>MPTFLLVNDDGYFSPGINALREALKSLGRVVVVAPDRNLSGVGHSLTFTEPLKMRKIDTDFYTVIDGTPADCVHLGYRVILEEKKPDLVLSGINEGPNLGEDITYSGTVSGAMEGRILGIPSIAFSAFGRENIMFEEIAKVCVDIVKKVLNEGIPEDTYLNVNIPNLRYEEIKGIKVTRQGKRA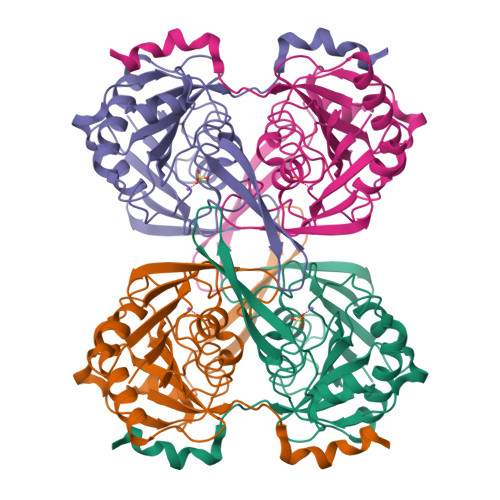YKERVFKYIDPYGKPFYWIAAEEFGWHAEEGTDYWAVLNGYVSVTPLHLDLTNYKVMKSIKYLEDSP[2x]> GSHSWRHIRAEGLDSSYTVLFGKAEADEIFQELEKEVEYFTGALARVQVFGKWHSVPRKQATYGDAGLTYTFSGLTLSPKPWIPVLERIRDHVSGVTGQTFNFVLINRYKDGSD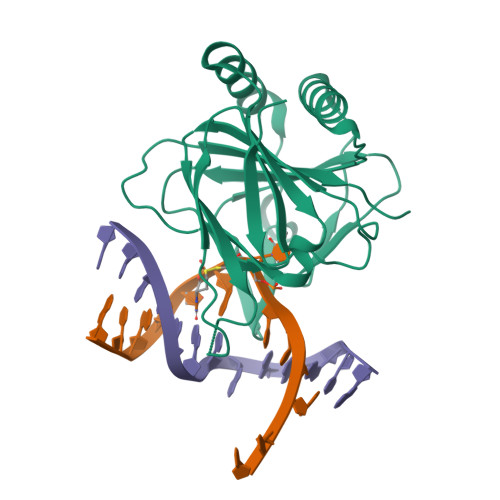HICEHRDDERELAPGSPIASVSFGASRDFVFRHKDSRGKSPSRRVAVVRLPLAHGSLLMMNHPTNTHWYHSLPVRKKVLAPRVNLTFRKILLTKK> MENSSKEDYKIQSFDLETQKLLKTALKDPGSVDLEKVSSVIVDQSLKDQVFSREAGRICYTIV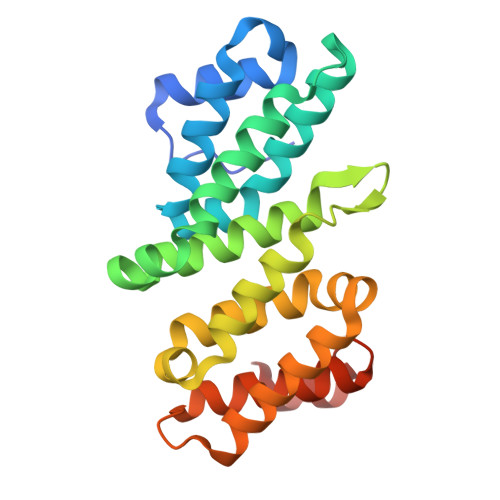QAEAKQTNGSVFRRNLLNRLQQEFKAREETRKRSTQEWVCLVSFICNIFDYLKVNNMPMVALVHPVYDCLFRLAQSDALKNEEEVDCLVLQLHRIGDQLEKMNVQLMDELFNLLRDGFLLQEDLSSMGRLLLLEILEFRAGGWKLSDTAQKYYYSEVTD> AGWNAYIDNLMADGTCQDAAIVGYKDSPSVWAAVPGKTFVNITPAEVGV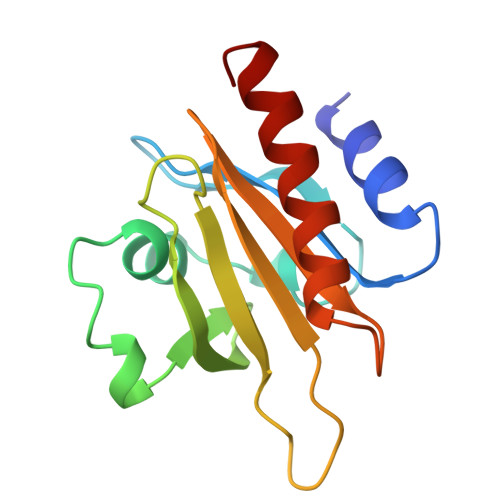LVGKDRSSFYVNGLTLGGQKCSVIRDSLLQDGEFSMDLRTKSTGGAPTFNVTVTKTDKTLVLLMGKEGVHGGLINKKCYEMASHLRRSQY>[2x]GPTEGEAGELRIAVESHTSFDWL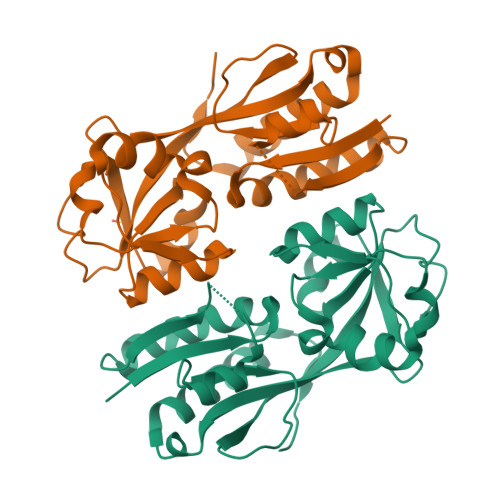MPAMGEFRPMWPQVELDIVSGFQADPVGLLLQHRADLAIVSEAEKQNGISFQPLFAYEMVGICAPDHPLAAKNVWTAEDFIGETLITYPVPDEMLDLPKKILIPKNINPPRRHSELTIAIIQLVASRRGIAALPYWTVMPYLEKGYVVHRQITADGLQSKLYAAIRTEDTDKSYLNNFCQIIRERGFADLPGLSELEPV> GSSGSSGMAFSGSQAPYLSPAVPFSGTIQGGLQDGLQITVNGTVLSSSGTRFAVNFQTGFSGNDIAFHFNPRFEDGGYVVCNTRQNGSWGPEERKTHMPFQKGMPFDLCFLVQSSDFKVMVNGILFVQYFHRVPFHRVDT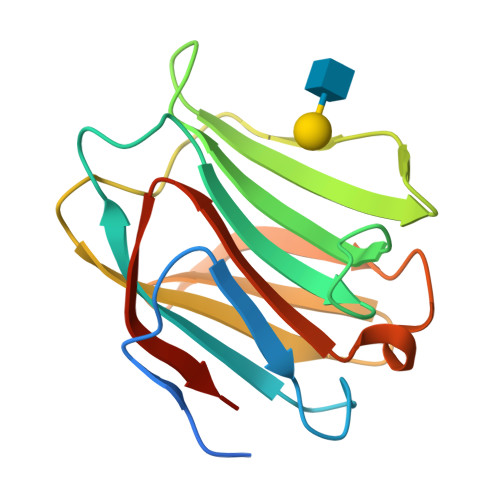ISVNGSVQLSYISFSGPSSG> VTNVGEDGEPGETEPRHALSPVDMHVHTDVSFLLDRFFDVETLELSNLTGSPATHVLDPFGSTAQLAWARLLNTCTYFFSDLELSIQFKFTTTPSSVGEGFVWVKWFPVGAPTKTTDAWQLEGGGNSVRIQQLAVAGMSPTVVFKIAGSRSQACGFSVPYTSMWRVVPVFYNGWGAPTKEKATYNWLPGAHFGSILLTSDAHDKGGCYLRYRFPRANMYCPRPIPPAFTRPADKTRHKFPTNINKQ;> DKKTEETTNIEDRIETTVVGVTIINSQGSVGTTYCYSKPDGRPPSTVSDPVTRLGPTLSRHYTFKVGEWPHSQSHGHAWICPLPSDKLKKMGSFHEVVKAHHLVKNGWDVVVQVNASFAHSGALCVAAVPEYEHTHEKALKWSELEEPAYTYQQLSVFPHQLLNLRTNSSVHLVMPYIGPGPTTNLTLHNPWTIVILILSELTGPGQTVPVTMSVAPIDAMVNGPLPNPE;> APIRVVSVPESDSFMSSVPDNSTPLYPKVVVPPRQVPGRFTNFIDVAKQTYSFCSISGKPYFEVTNTSGDEPLFQMDVSLSAAELHGTYVASLSSFFAQYRGSLNFNFIFTGAAATKAKFLVAFVPPHSAAPKTRDEAMACIHAVWDVGLNSAFSFNVPYSSPADFMAVYSAEATVVNVSGWLQVYALTALTSTDIAVNSKGRVLVAVSAGPDFSLRHPVDLPDKQ;> GAGTSTPTTGNQNMSGNSGSIVQNFYMQQYQNSIDADLGDNVISPEGQGSNTSSSTSSSQSSGLGGWFSSLLNLGTKLLA

Equine rhinitis A virus (ERAV) shares physicochemical properties such as buoyant density, base composition and acid lability with foot-and-mouth-disease virus (FMDV). The mature capsid comprises 60 copies of each of four proteins: VP1-4 (with molecular weights of 25, 25, 22 and 11 kDa respectively for ERAV). VP1-3 are composed of eight-stranded β-sandwiches, with strands denoted CHEF and BIDG respectively on the two sheets, which form a pseudo T = 3 icosahedral lattice with the CHEF sheet exposed on the capsid surface and BIDG to the interior. To investigate how similar ERAV and FMDV are in terms of structure and to probe further the cell entry mechanism for aphthoviruses we have determined crystal structures of ERAV at two different pHs, using highly optimised methods since the yield of purified virus was very low.

Crystals grown at neutral pH only yielded poor, incomplete data to 3.5 Å but possessed 120-fold non-crystallographic symmetry. Averaging rendered the electron density clear, delineated differences on the inside of the capsid compared to the low pH structure, and confirmed that there were no major changes elsewhere in the particle. A structure–based phylogenetic tree constructed from similarities between the biological protomers of picornaviruses indicates that ERAV is most similar to FMDV. In contrast the surface profile for ERAV extends to an outer radius of 159 Å at a prominent crown around the five-fold axis built from the extended VP1 loops (Mengo virus has an outer radius of 164 Å). The ERAV structure reveals the presence of capsid pores similar to those seen in FMDV, at the 5-fold and 3-fold axes of symmetry. Residues 14–27 form a hairpin contributing to an extended β-sheet which stabilizes the pentamer interface. In FMDVs the protonation of a cluster of histidine residues (pI = 7.8) at the interface acts as a switch to dissociate the pentamers below pH 7, whilst ERAV, which in the native structure follows the canonical FMDV interface structure, has fewer histidines, consistent with the somewhat lower pH at which it dissociates into pentamers (between pH 6.5 and 5.5). The similarity between the two structures extends to the calcium ions bound on the icosahedral 3-fold axes (liganded by Asp 195 and Thr 194 of VP3) in both the low pH and native particles. Similarly, there are no alterations in the ERAV pores between the low-pH and native structures to support their involvement in the exit of the genome.>[7x]MAIAHIATEYVFSDFLLKDPPESKYKGLRLELAVDKLVSCIAVGLPLLLISLAFAQEITLGSQISCFAPTSFSWRQAAYVDSFCWAAVQQKHLSQSDSGNVPLWLHKFFPYILLLVAVLLYLPNLFWRFTAAPHLSSDLKFVMEELDKCYNRDIK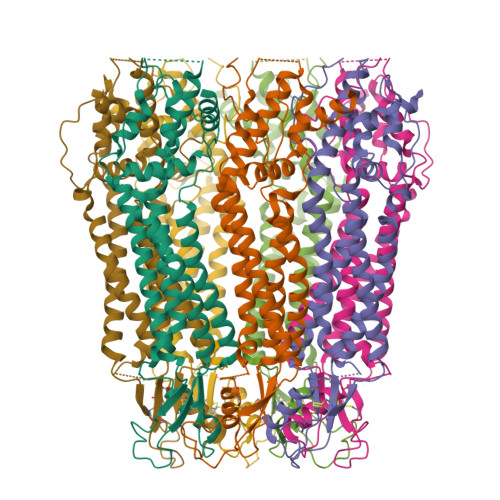DIKAANNLNSSDKRDYPIVEQYLKTKNNSYGLIIKYLICRVVTLIIVFTACIYLGYYISLFSLTDEFTCNIRTGILRNDTALPPLVQCKLIAVGVFRLLSYINLIIYVLIMPFIIYAMLVPFRKTANVLKVYEVLPTFSVQQAPSKTYDDHSLFLLFLEENVSELKSYKFLKVLENIKASSWSHPQFEK>PEENTLATAKEQGDEQEWSLILVNRQNPIPAQYDVELEQLSNGERIDIRISPYLQDLFDAARADGVYPIVASGYRTTEKQQEIMDEKVAEYKAKGYTSAQAKAAAETWVAVPGTSEHQLGLAVDINADGIHSTGNEVYRWLDENSYRFGFIRRYPPDKTEI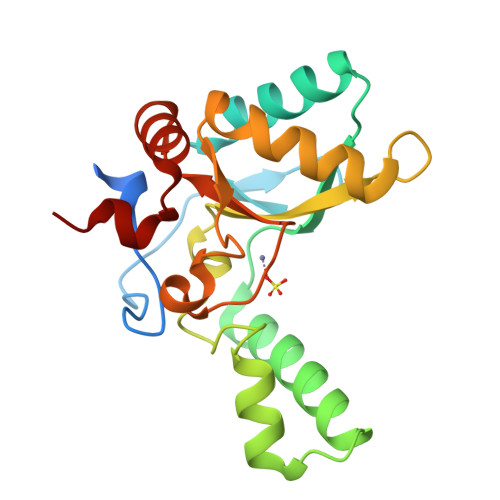TGVSNEPWHYRYVGIEAATKIYHQGLCLEEYLNTEK[6x]(4aP)-N,N-diethyl-9,9-dimethyl-7-[(1E)-prop-1-en-1-yl]-9H-fluoren-2-amine | C22 H27 N | 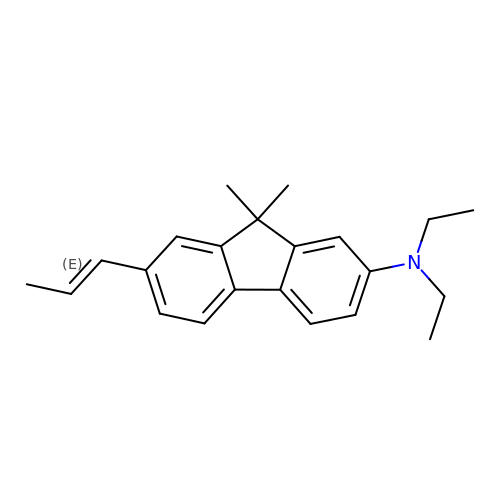UMARKYXLRJLTSK-RMKNXTFCSA-N> GMNLQTDQTTTTADESAIRAFHRQMIDAWNRGSGEG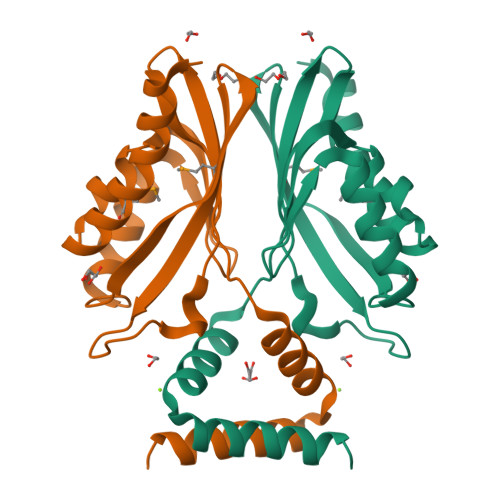FAAPFSETADFITFEGTHLKGRKEIAAFHQQAFDTVVKGTRLEGEVDFVRFVNSQLALMLVVIRVILPGQTETSASRDSLPLYVVTKGDEGWQIEGLLNTRKLTLERQFFLDDFDSLSAEAQRQVTDLVASLKQSH>[4x]GSPASGTSLSAAIHRTQLWFHGRISREESQRLIGQQGLVDGLFLVRESQRNPQGFVLSLCHLQKVKHYLILPSEEEGRLYFSMDDGQTRFTDLLQLVEFHQLNRGILPCLL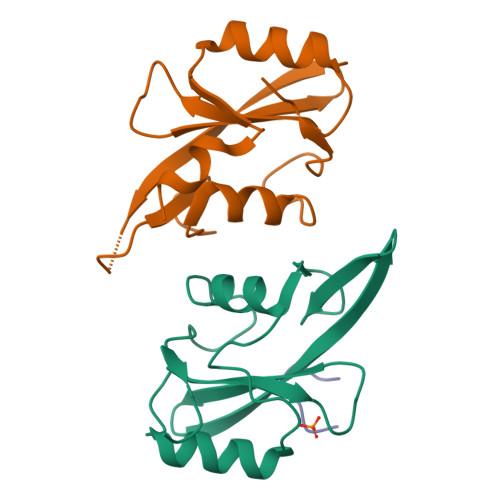RHCCTRVAL;>SFEGYDNSC[2x]>DHY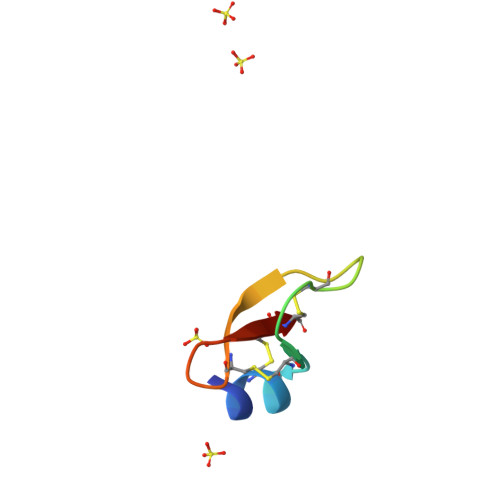NCVSSGGQCLYSACPIFTKIEGTCYRGKAKCCK[4x]> MELRHTPARDLDKFIEDHLLPNTCFRTQVKEAIDIVCRFLKERCFQGTADPVRVSKVVKGGSSGKGTTLRGRSDADLVVFLTKLTSFEDQLRRRGEFIQEIRRQLEACQREQKFKVTFEVQSPRRENPRALSFVLSSPQLQQEVEFDVRP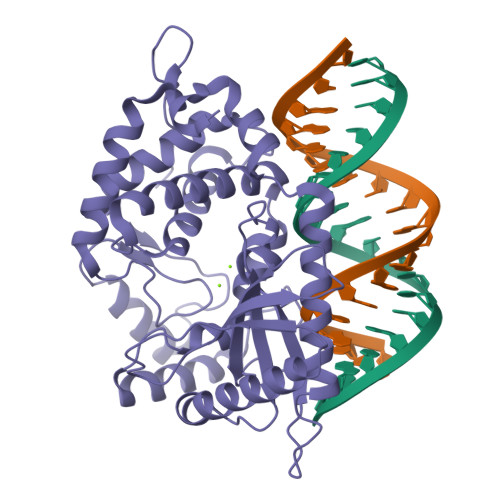AFDALGQWTPGYKPNPEIYVQLIKECKSRGKEGEFSTCFTELQRDFLRNRPTKLKSLIRLVKHWYQTCKKTHGNKLPPQYALELLTVYAWEQGSRKTDFSTAQGFQTVLELVLKHQKLCIFWEAYYDFTNPVVGRCMLQQLKKPRPVILDPADPTGNVGGGDTHSWQRLAQEARVWLGYPCCKNLDGSLVGAWTMLQKIGSHHHHHH>MGDGANSDAAKEYLTKDSFSYEVYGIIAMQAAYRDYDSGDAKQDDNLGGMQLNNESRIGFRGKKQFANFEPTFIWQIEGGYVDPSFGGEGAGLGERDTFVGFESASWGQVRLGRVLTPMYELVDWPASNPGLGDVYDWGGAIGGAKYQDRQSNTIRWDSPMYADKFSIDAAVGAGDKAGLGAGDDYWGGIAAHYKLGPLQLDAAYEGNRNIEAEGQTWENNTYLVGVQGWFENGISFFAQYKYMEADASNGVNEKQDAMSAGLMYTTGDWQYKLGYAANFDLERDGKTLSNTSDDVVSAQIMYFVDPSAVLYARARMNDFNEGLDGLDDAARWTSGT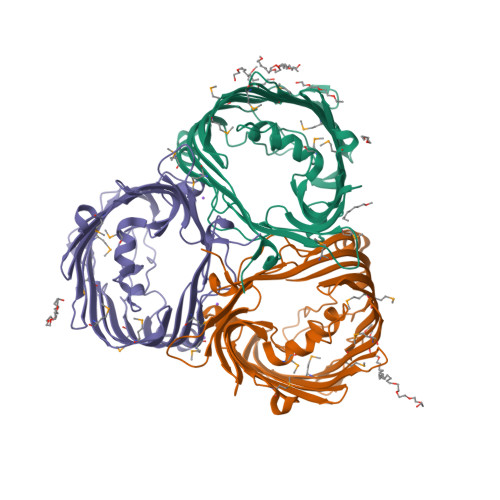NGDYNEYSVGVEYYF[6x]>[2x]GIKFSAEALRCHLRDHVNVSMVEVTDFPFNTSEWEGYLPKESIRTKAGPWGRCAVVSSAGSLKSSQLGREIDDHDAVLRFNGAPTANFQQDVGTKTTIRLMNSQLVTTEKRFLKDSLYNEGILIVWDPSVYHSDIPKWYQNPDYNFFNNYKTYRKLHPNQPFYILKPQMPWELWDILQEI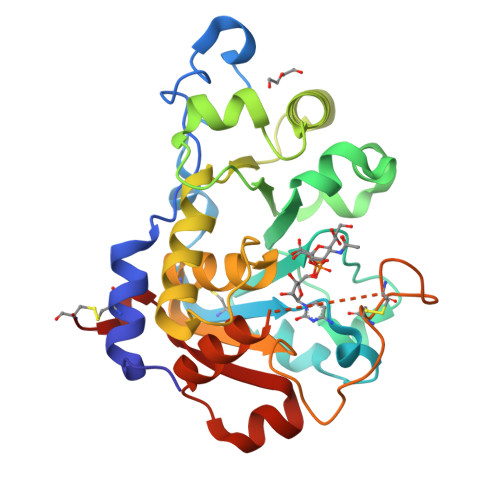SPEEIQPNPPSSGMLGIIIMMTLCDQVDIYEFLPSKRKTDVCYYYQKFFDSACTMGAYHPLLYEKNLVKHLNQGTDEDIYLLGKATLPGFRTIHC>GMSEPYTWKSVVTGAGGGFVPGIIFNQTEPNLIYARTDIGGAYRWNQATSSWVSISDSVGWVDWNKNGVDALATDPIDPNK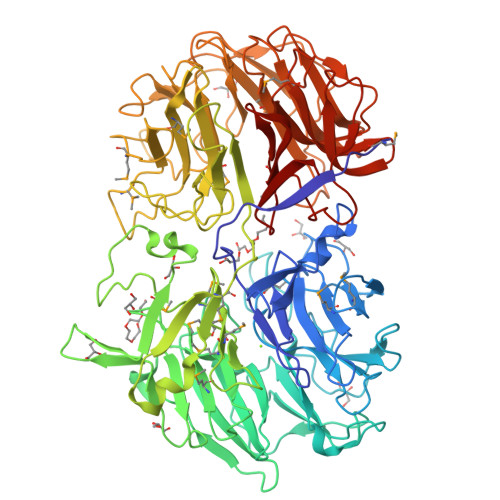VYMATGTYTNHWDNNGQIMRSNDRGNTWQTTPLPFKVGGNMPGRSAGERLVIDPNKNNILYFGARSGNGLWKSIDSGVTWSKVTSFPNVGTYIQNPTLDYGNDLVGLSWITFDKSTGTLGNATQTIYVGVADTASSVYRSTDGGVTWTALAGQPTGFLPHHGELSSTGDLYITYSNGVGPYDGSKGEVWKYNKTSGAWTNISPTTGTDNWYGFGGLALDAQHPNTLMVSSLNAWWPDEVIFRSTNGGATWSRIWDWGNYPERTYKFSMDITAAPWLDHGTTSTSLDPSPKLGWMMGDLEIDPFNSNRMMYGTGATIYGSNNLTSWDTGGKVNISVMAKGVEETAVLGLISPPTGTSHLITALGDVSGFRHEDLSVAPTKFQTSPSWATTMSIDYAELSPSYMVRVGSADKEKTPSMKSIGISNDGGVNWYMPNSEPSNGTKTTVGHGQVAVSASGNSILWSTSDIGVYYSKTSGNSWTASAGLPAGAKIASDRVNPNKYYGFYAGTFYVSVDGGATFTATGASGFPTNNVAGLQPNEAQISMKAVPGIEGDIWFAGGNTVENKYGLWHSTNSGASFTKLTNVEEADLIGYGKAAPGQTYMSLYTVAKIDGVRGVFRSDDVGATWVRINDDAHQYAKINMAITGDPRIYGRVYLGTNGRGTLYADPV[8x]> MSEQNNAVLPKGVTQGEFNKAVQKFRALLGDDNVLVESDQLVPYNKIMMPVENAAHAPSAAVTATTVEQVQGVVKICNEHKIPIWTISTGRNFGYGSAAPVQRGQVILDLKKMNKIIKIDPEMCYALVEPGVTFGQMYDYIQENNLPVMLSFSAPSAIAGPVGNTMDRGVGYTPYGEHFMMQCGMEVVLANGDVYRTGMGGVPGSNTWQIFKWGYGPTLDGMFTQANYGICTKMGFWLMPKPPVFKPFEVIFEDEADIVEIVDALRPLRMSNTIPNSVVIASTLWEAGSAHLTRAQYTTEPGHTPDSVIKQMQKDTGMGAWNLYAALYGTQEQVDVNWKIVTDVFKKLGKGRIVTQEEAGDTQPFKYRAQLMSGVPNLQEFGLYNWRGGGGSMWFAPVSEARGSECKKQAAMAKRVLHKYGLDYVAEFIVAPRDMHHVIDVLYDRTNPEETKRADACFNELLDEFEKEGYAVYRVNTRFQDRVAQSYGPVKRKLEHAIK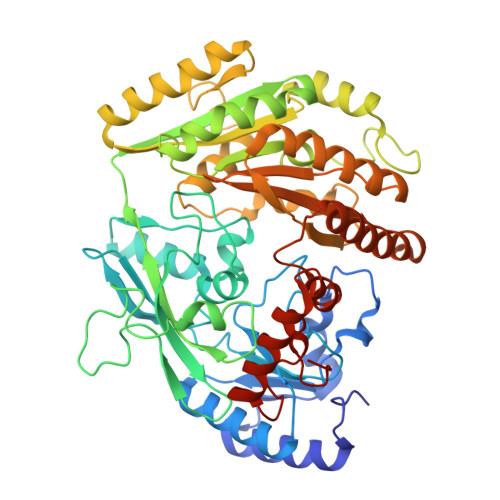RAVDPNNILAPGRSGIDLNNDF> XXXXXXXXXXXXXXXXXXXXXXXXXXXXXXXXXXXXXXXXXXXXXXXXXXXXXXXXXXXXXXXXXXXXXXXXXXXXXXXXXXXXXXXXXXXXXXXXXXXXXXXXXXXXXXXXXXXXXXXXXXXXXXXXXXXXXXXXXXXXXXXXXXXXXXXXXXXXXXXXXXXXXXXXXXXXXXXXXXXXXX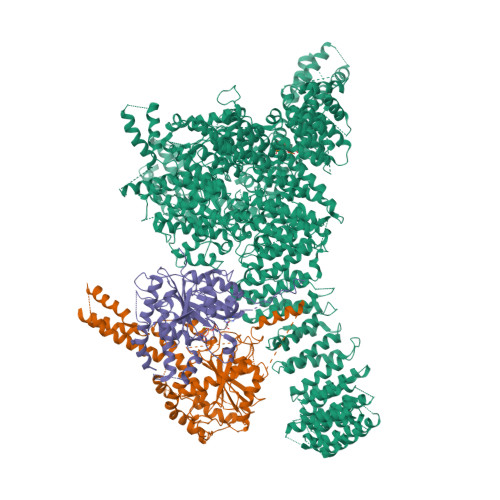XXXXXXXXXXXXXXXXXXXXXXXXXXXXXXXXXXXXXXXXXXXXXXXXXXXXXXXXXXXXXXXXXXXXXXXXXXXXXXXXXXXXXXXXXXXXXXXXXXXXXXXXXXXXXXXXXXXXXXXXXXXXXXXXXXXXXXXXXXXXXXXXXXXXXXXXXXXXXXXXXXXXXXXXXXXXXXXXXXXXFSTNFRDTVDILVGWHIDHTQKPSLTQQVSGWLQSLEPFWVADLAFSTTLLGQFLEDMEAYAEDLSHVASGESVDEDVPPPSVSLPKLAALLRVFSTVVRSIGERFSPIRGPPITEAYVTDVLYRVMRCVTAANQVFFSEAVLTAANECVGVLLGSLDPSMTIHCDMVITYGLDQLENCQTCGTDYIISVLNLLTLIVEQINTKLPSSFVEKLFIPSSKLLFLRYHKEKEVVAVAHAVYQAVLSLKNIPVLETAYKLILGEMTCALNNLLHSLQLPEACSEIKHEAFKNHVFNVDNAKFVVIFDLSALTTIGNAKNSLIGMWALSPTVFALLSKNLMIVHSDLAVHFPAIQYAVLYTLYSHCTRHDHFISSSLSSSSPSLFDGAVISTVTTATKKHFSIILNLLGILLKKDNLNQDTRKLLMTWALEAAVLMRKSETYAPLFSLPSFHKFCKGLLANTLVEDVNICLQACSSLHALSSSLPDDLLQRCVDVCRVQLVHSGTRIRQAFGKLLKSIPLDVVLSNNNHTEIQEISLALRSHMSKAPSNTFHPQDFSDVISFILYGNSHRTGKDNWLERLFYSCQRLDKRDQSTIPRNLLKTDAVLWQWAIWEAAQFTVLSKLRTPLGRAQDTFQTIEGIIRSLAAHTLNPDQDVSQWTTADNDEGHGNNQLRLVLLLQYLENLEKLMYNAYEGCANALTSPPKVIRTFFYTNRQTCQDWLTRIRLSIMRVGLLAGQPAVTVRHGFDLLTEMKTTSLSQGNELEVTIMMVVEALCELHCPEAIQGIAVWSSSIVGKNLLWINSVAQQAEGRFEKASVEYQEHLCAMTGVDCCISSFDKSVLTLANAGRNSASPKHSLNGESRKTVLSKPTDSSPEVINYLGNKACECYISIADWAAVQEWQNAIHDLKKSTSSTSLNLKADFNYIKSLSSFESGKFVECTEQLELLPGENINLLAGGSKEKIDMKKLLPNMLSPDPRELQKSIEVQLLRSSVCLATALNPIEQDQKWQSITENVVKYLKQTSRIAIGPLRLSTLTVSQSLPVLSTLQLYCSSALENTVSNRLSTEDCLIPLFSEALRSCKQHDVRPWMQALRYTMYQNQLLEKIKEQTVPIRSHLMELGLTAAKFARKRGNVSLATRLLAQCSEVQLGKTTTAQDLVQHFKKLSTQGQVDEKWGPELDIEKTKLLYTAGQSTHAMEMLSSCAISFCKSVKAEYAVAKSILTLAKWIQAEWKEISGQLKQVYRAQHQQNFTGLSTLSKNILTLIELPSVNTMEEEYPRIESESTVHIGVGEPDFILGQLYHLSSVQAPEVAKSWAALASWAYRWGRKVVDNASXXXXXXXXXXXXXXXXXXXXXXXXXXXXXXXXXXXXXXXXXXXXXXXXXXXXXXXXXXXXXXXXXXXXXXXXXXXXXXXXXXXXXXXXEGVIKVWRKVVDRIFSLYKLSCSAYFTFLKLNAGQIPLDEDDPRLHLSHRVEQSTDDMIVMATLRLLRLLVKHAGELRQYLEHGLETTPTAPWRGIIPQLFSRLNHPEVYVRQSICNLLCRVAQDSPHLILYPAIVGTISLSSESQASGNKFSTAIPTLLGNIQGEELLVSECEGGSPPASQDSNKDEPKSGLNEDQAMMQDCYSKIVDKLSSANPTMVLQVQMLVAELRRVTVLWDELWLGVLLQQHMYVLRRIQQLEDEVXXXXXXXXXXXXXXXXXXXXXXXXXXXXXXXXXXXXXXXXXXXXXXPHEKWFQDNYGDAIENALEKLKXXXXXXXXXXXXXXXXXXXXXXXXXXXXXXYILRLEEISPWLAAMTNTEIALPGEVSARDTVTIHSVGGTITILPTKTKPKKLLFLGSDGKSYPYLFKGLEDLHLDERIMQFLSIVNTMFATINRQETPRFHARHYSVTPLGTRSGLIQWVDGATPLFGLYKRWQQREAALQAQKXXXXXXXXXXXXXXXXXXXXXXXXXXXXXXXXXXXXXXXXXXWPLHVMKAVLEELMEATPPNLLAKELWSSCTTPDEWWRVTQSYARSTAVMSMVGYIIGLGARHLDNVLIDMTTGEVVHIDYNVCFEKGKSLRVPEKVPFRMTQNIETALGVTGVEGVFRLSCEQVLHIMRRGRETLLTLLEAFVYDPLVDWTAGGEAGFAGAVYGGGGQQAESKQSKREMEREITRSLFSSRVAEIKVNWFKNRDEMLVVLPKLDGSLDEYLSLQEQLTDVEKLQGKLLEEIEFLEGAEGVDHPSHTLQHRYSEHTQLQTQQRAVQEAIQVKLNEFEQWITHYQAAFNNLEATQLASLLQEISTQMDLGPPSYVPATAFLQNAGQAHLISQCEQLEGEVGALLQQRRSVLRGCLEQLHHYATVALQYPKAIFQKHRIEQWKTWMEELICNTTVERCQELYRKYEMQYAPQPPPTVCQFITATEMTLQRYAADINSRLIRQVERLKQEAVTVPVCEDQLKEIERCIKVFLHENGEEGSLSLASVIISALCTLTRRNLMMEGAASSAGEQLVDLTSRDGAWFLEELCSMSGNVTCLVQLLKQCHLVPQDLDIPNPMEASETVHLANGVYTSLQELNSNFRQIIFPEALRCLMKGEYTLESMLHELDGLIEQTTDGVPLQTLVESLQAYLRNAAMGLEEETHAHYIDVARLLHAQYGELIQPRNGSVDETPKMSAGQMLLVAFDGMFAQVETAFSLLVEKLNKMEIPIAWRKIDIIREARSTQVNFFDDDNHRQVLEEIFFLKRLQTIKEFFRLCGTFSKTLSGSSSLEDQNTVNGPVQIVNVKTLFRNSCFSEDQMAKPIKAFTADFVRQLLIGLPNQALGLTLCSFISALGVDIIAQVEAKDFGAESKVSVDDLCKKAVEHNIQIGKFSQLVMNRATVLASSYDTAWKKHDLVRRLETSISSCKTSLQRVQLHIAMFQWQHEDLLINRPQAMSVTPPPRSAILTSMKKKLHTLSQIETSIATVQEKLAALESSIEQRLKWAGGANPALAPVLQDFEATIAERRNLVLKESQRASQVTFLCSNIIHFESLRTRTAEALNLDAALFELIKRCQQMCSFASQFNSSVSELELRLLQRVDTGLEHPIGSSEWLLSAHKQLTQDMSTQRAIQTEKEQQIETVCETIQNLVDNIKTVLTGHNRQLGDVKHLLKAMAKDEEAALADGEDVPYENSVRQFLGEYKSWQDNIQTVLFTLVQAMGQVRSQEHVEMLQEITPTLKELKTQSQSIYNNLVSFASPLVTDATNECSSPTSSATYQPSFAAAVRSNTGQKTQPDVMSQNARKLIQKNLATSADTPPSTVPGTGKSVACSPKKAVRDPKTGKAVQERNSYAVSVWKRVKAKLEGRDVDPNRRMSVAEQVDYVIKEATNLDNLAQLYEGWTAWV;> MAGPVSLRDLLMGASAWMGSESPGGSPTEGGGSAAGGPEPPWREDEICVVGIFGKTALRLNSEKFSLVNTVCDRQVFPLFRHQDPGDPGPGIRTEAGAVGEAGGAEDPGAAAGGSVRGSGAVAEGNRTEAGSQDYSLLQAYYSQESKVLYLLLTSICDNSQLLRACRALQSGEAGGGLSLPHAEAHEFWKHQEKLQCLSLLYLFSVCHILLLVHPTCSFDITYDRVFRALDGLRQKVLPLLKTAIKDCPVGKDWKLNCRPCPPRLLFLFQLNGALKVEPPRNQDPAHPDKPKKHSPKRRLQHALEDQIYRIFRKSRVLTNQSINCLFTVPANQAFVYIVPGSQEEDPVGMLLDQLRSHCTVKDPESLLVPAPLSGPRRYQVMRQHSRQQLSFHIDSSSSSSSGQLVDFTLREFLWQHVELVLSKKGFDDSVGRNPQPSHFELPTYQKWISAASKLYEVAIDGKEEDLGSPTGELTSKILSSIKVLEGFLDIDTKFSENRCQKALPMAHSAYQSNLPHNYTMTVHKNQLAQALRVYSQHARGPAFHKYAMQLHEDCYKFWSNGHQLCEERSLTDQHCVHKFHSLPKSGEKPEADRNPPVLYHNSRARSTGACNCGRKQAPRDDPFDIKAANYDFYQLLEEKCCGKLDHINFPVFEPSTPDPAPAKNESSPAPPDSDADKLKEKEPQTQGESTSLSLALSLGQSTDSLGTYPADPQAGGDNPEVHGQVEVKTEKRPNFVDRQASTVEYLPGMLHSNCPKGLLPKFSSWSLVKLGPAKSYNFHTGLDQQGFIPGTNYLMPWDIVIRTRAEDEGDLDTNSWPAPNKAIPGKRSAVVMGRGRRRDDIARAFVGFEYEDSRGRRFMCSGPDKVMKVMGSGPKESALKALNSDMPLYILSSSQGRGLKPHYAQLMRLFVVVPDAPLQIILMPQVQPGPPPCPVFYPEKQEITLPPDGLWVLRFPYAYVTERGPCFPPKENVQLMSYKVLRGVLKAVTQ;> MSESGHSQPGLYGIERRRRWKEPGSGGPQNLSGPGGRERDYIAPWERERRDASEETSTSVMQKTPIILSKPPAERSKQPPPPTAPAAPPAPAPLEKPIVLMKPREEGKGPVAVTGASTPEGTAPPPPAAPAPPKGEKEGQRPTQPVYQIQNRGMGTAAPAAMDPVVGQAKLLPPERMKHSIKLVDDQMNWCDSAIEYLLDQTDVLVVGVLGLQGTGKSMVMSLLSANTPEEDQRTYVFRAQSAEMKERGGNQTSGIDFFITQERIVFLDTQPILSPSILDHLINNDRKLPPEYNLPHTYVEMQSLQIAAFLFTVCHVVIVVQDWFTDLSLYRFLQTAEMVKPSTPSPSHESSSSSGSDEGTEYYPHLVFLQNKARREDFCPRKLRQMHLMIDQLMAHSHLRYKGTLSMLQCNVFPGLPPDFLDSEVNLFLVPFMDSEAESENPPRAGPGSSPLFSLLPGYRGHPSFQSLVSKLRSQVMSMARPQLSHTILTEKNWFHYAARIWDGVRKSSALAEYSRLLA>[2x]SPEFMVKAKSWTLKKHFQGKPTQSDFELKTVELPPLKNGEVLLEALFLSVDPYMRIASKRLKEGAVMMGQQVARVVESKNSAFPAGSIVLAQSGWTTHFISDGKGLEKLLTEWPDKLPLSLALGTIGMPGLTAYFGLLEVCGVKGGETVLVSAAAGAVGSVVGQIAKLKGCKVVGAAGSDEKIAYLKQIGFDAAFNYKTVNSLEEALK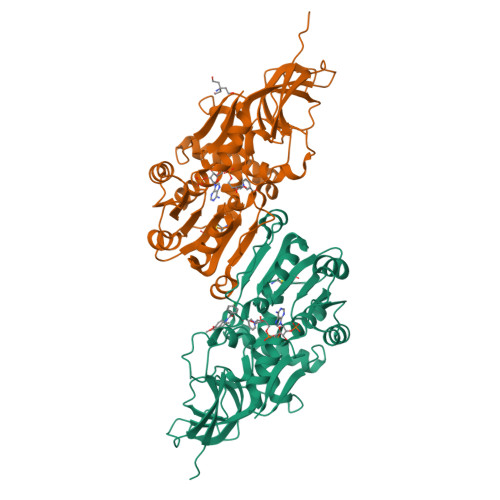KASPDGYDCYFDNVGGEFLNTVLSQMKDFGKIAICGAISVYNRMDQLPPGPSPESIIYKQLRIEGFIVYRWQGDVREKALRDLMKWVLEGKIQYHEHVTKGFENMPAAFIEMLNGANLGKAVVTA Within this class of proteins, the bromodomain and extraterminal domain (BET) family contains four members that are transcriptional coregulators and that recognize acetyllysines (AcKs) using a tandem pair of highly homologous bromodomains (BDs). Despite heavy academic and industry investment in this area, the generation of paralog-selective inhibitors has proved elusive because of the extremely high sequence similarity between the bromodomains of family members (90 to 95% within the acetyllysine-binding pocket residues). Using the highly conserved BET BDs as a model system, we conducted three mRNA display-based RaPID (random nonstandard peptides integrated discovery) screens using a single library (which contains >1012 unique members). Crystal structures of 13 distinct peptide–bromodomain complexes revealed highly diverse structures and binding modes among the cyclic peptide ligands.

In contrast to our observations for peptide 3.1C, where selectivity between BD1- and BD2-type domains appears to derive from contacts in a region distal to the AcK pocket, the 3.1B peptide recognizes the BD2 domain in a very different manner. The peptide and BD form a 1:1 complex in which it is AcK5 that is bound in the pocket (cf. AcK12 in interactions with BD1 domains). In this case, the interaction surface area is much smaller than observed for the BRD4-BD1 structure, consistent with the substantially lower KD. Furthermore, CSPs observed upon addition of 3.1B to 15N-labeled BRD2-BD2 are consistent with this binding mode, indicating that this peptide binds to all BD2 domains in the same manner. This difference again highlights the ability of RaPID-selected peptides to robustly distinguish BD1- from BD2-type domains.

> QGPLGSSKVSEQLKCCSGILKEMFAKKHAAYAWPFYKPVDVEALGLHDYCDIIKHPMDMSTIKSKLEAREYRDAQEFGADVRLMFSNCYKYNPPDHEVVAMARKLQDVFEMRFAKMPDEPEEP;> XWKTIKGKTWRTKQC>MSLFKIRMPETVAEGTRLALRAFSLVVAVDEHGGIGDGRSIPWNVPEDMKFFRDLTTKLRGKNVKPSPAKRNAVVMGRKTWDSIPPKFRPLPGRLNVVLSSTLTTQHLLDGLPDEEKRNLHADSIVAVNGGLEQALRLLASPNYTPSIETVYCIGGGSVYAEALRPPCVHLLQAIYRTTIRASESSCSVFFRVPESGTEAAAGIEWQRETISEELTSANGNETKYYFEKLIPRNREEEQYLSLVDRIIREGNVKHDRTGVGTLSIFGAQMRFSLRNNRLPLLTTKRVFWRGVCEELLWFLRGETYAKKL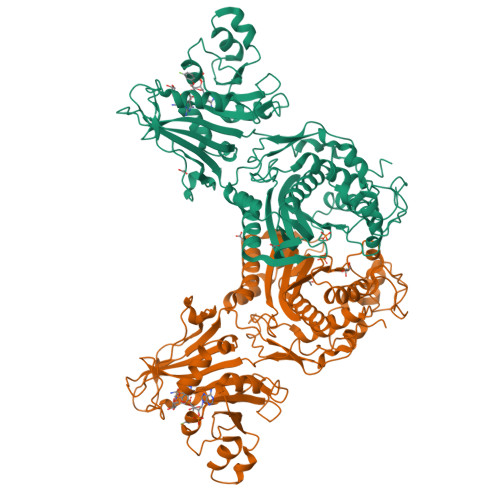SDKGVHIWDDNGSRAFLDSRGLTEYEEMDLGPVYGFQWRHFGAAYTHHDANYDGQGVDQIKAIVETLKTNPDDRRMLFTAWNPSALPRMALPPCHLLAQFYVSNGELSCMLYQRSCDMGLGVPFNIASYALLTILIAKATGLRPGELVHTLGDAHVYSNHVEPCNEQLKRVPRAFPYLVFRREREFLEDYEEGDMEVIDYAPYPPISMKMAV[4x]> MSHPDYRMNLRPLGTPRGVSAVAGPHDIGASPGDKKSKNRSTRGKKKSIFETYMSKEDVSEGLKRGTLIQGVLRINPKKFHEAFIPSPDGDRDIFIDGVVARNRALNGDLVVVKLLPEEHWKVVKPESNDKETEAAYESDIPEELCGHHLPQQSLKSYNDSPDVIVEAQFDGSDSEDGHGITQNVLVDGVKKLSVCVSEKGREDGDAPVTKDETTCISQDTRALSEKSLQRSAKVVYILEKKHSRAATGFLKLLADKNSELFRKYALFSPSDHRVPRIYVPLKDCPQDFVARPKDYANTLFICRIVDWKEDCNFALGQLAKSLGQAGEIEPETEGILTEYGVDFSDFSSEVLECLPQGLPWTIPPEEFSKRRDLRKDCIFTIDPSTARDLNDALSCKPLADGNFKVGVHIADVSYFVPEGSDLDKVAAERATSVYLVQKVVPMLPRLLCEELCSLNPMSDKLTFSVIWTLTPEGKILDEWFGRTIIRSCTKLSYEHAQSMIESPTEKIPAKELPPISPEHSSEEVHQAVLNLHGIAKQLRQQRFVDGALRLDQLKLAFTLDHETGLPQGCHIYEYRESNKLVEEFMLLANMAVAHKIHRAFPEQALLRRHPPPQTRMLSDLVEFCDQMGLPVDFSSAGALNKSLTQTFGDDKYSLARKEVLTNMCSRPMQMALYFCSGLLQDPAQFRHYALNVPLYTHFTSPIRRFADVLVHRLLAAALGYRERLDMAPDTLQKQADHCNDRRMASKRVQELSTSLFFAVLVKESGPLESEAMVMGILKQAFDVLVLRYGVQKRIYCNALALRSHHFQKVGKKPELTLVWEPEDMEQEPAQQVITIFSLVEVVLQAESTALKYSAILK

Dis3-like 2 (Dis3L2) is a 3′–5′ exoribonuclease that plays a critical role in human development. Dis3L2 independently degrades structured substrates, including coding and noncoding 3′ uridylated RNAs. Unlike a number of structurally similar homologs, Dis3L2 can degrade structured RNAs independent of external helicase activity. We determined the structures of an RNase R/II family nuclease bound to a series of structured RNA substrates and analyzed the kinetic profiles of wild-type Homo sapiens Dis3L2 (HsDis3L2) and engineered mutants to reveal how this nuclease achieves highly efficient degradation of structured RNA.

To understand the presubstrate binding state, we used cryogenic electron microscopy (cryo-EM) to determine the structure of RNA-free HsDis3L2 to 3.4 Å resolution (construct Dis3L2D391N residues 1–858: carboxy (C)-terminal truncation of residues 859–885; and an engineered catalytic mutation of Asp for Asn at residue 391 in Dis3L2). RNA-free HsDis3L2 has a vase-like conformation in which three oligonucleotide/oligosaccharide-binding (OB) domains—two cold shock domains (CSDs) and an S1 domain—encircle a funnel-like tunnel that reaches into the Ribonuclease B (RNB) domain and leads to the active site. The OB domains provide a large positively charged surface, which probably acts as a landing pad for the negatively charged RNA. The overall structure of RNA-free Dis3L2 is very similar to the structure of the mouse Dis3L2–ssRNA complex (MmDis3L2–U13) (root mean square deviation (RMSD) = 1.2 Å, calculated over all Cα pairs). Thus, the apoenzyme is preorganized to bind single-stranded RNA (ssRNA). The vase conformation is the only one observed in the RNA-free form and with long single-stranded 3′ overhangs. RNA-free Dis3L2 is preorganized in a vase conformation to bind RNA substrates (yellow), with a seven-nucleotide-deep tunnel leading to the nuclease active site.> SRLNRESVIDAALELLNETGIDGLTTRKLAQKLGIEQPTLYWHVKNKRALLDALAVEIL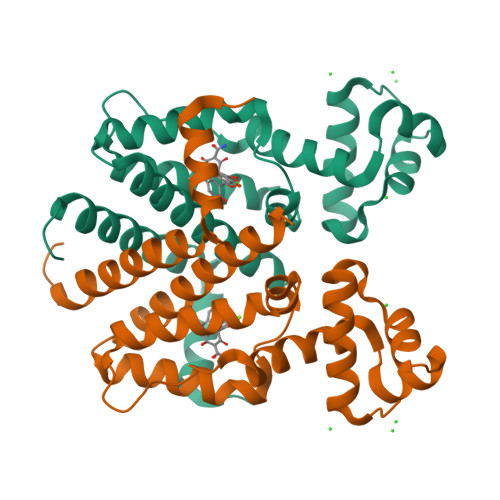ARHHDYSLPAAGESWQSFLRNNAMSFRRALLRYRDGAKVHLGARPDEKQYDTVETQLRFMTENGFSLRDGLYAISAVSHFTLGAVLEQQEHTAALTDRPAAPDENLPPLLREALQIMDSDDGEQAFLHGLESLIRGFEVQLTALLQIV>[2x]TNKELQAIRKLLMLDVSEAAEHIGRVSARSWQYWESGRSAVPDDVEQEMLDLASVRIEMMSAIDKRLADGERPKLRFYNKLDEYLADNPDHNVIGWRLSQSVAALYYTEGHADLI

Bacteria are under constant threat of invasion by bacteriophages (phages) and other mobile genetic elements (MGEs). Among the many protection strategies employed against these invaders, the highly diverse CRISPR-Cas systems stand out as the only known adaptive immune systems in bacteria.

Here, we report the first structure of an Aca protein, the Aca2 DNA-binding transcriptional autorepressor from Pectobacterium carotovorum bacteriophage ZF40, determined to 1.34 Å. Aca2 presents a conserved N-terminal helix-turn-helix DNA-binding domain and a previously uncharacterized C-terminal dimerization domain. The elution volume during the final size exclusion chromatography run indicated that the 13.7 kDa Aca2 protein forms a dimer in solution, corroborating what was observed with our previous constructs. The Aca2 dimer structure shows each protomer stacked against one another in opposition, like the letter X, such that the HTH motifs are aligned along the “base” of the dimer. Examining a single protomer shows that the proposed NTD HTH and relative C-terminal domain (CTD) are in fact small clusters of secondary structure elements abutting and joined by a longer backbone α-helix, α4, such that the protomer forms a single globular protein. Whilst the NTD provides the HTH motif for DNA-binding, the CTD stabilizes the positioning of the NTD from the other protomer by stacking α6 against the other protomer α1, thereby aiding dimerization. The Aca2 protomer-protomer interface was analyzed using PDBsum, which calculated a buried surface area of 1213 Å2. This is supported by two salt bridges formed between R57 within α4 of protomer A and E110 within α6 of protomer B, and vice versa. Whilst the upper CTD surface of the dimer contains mixed patches of both electropositive and electronegative potential, the NTD HTH motif is clearly electropositive and primed for DNA binding (left). Dimerization positions the Aca2 recognition helices for insertion into the major grooves of target DNA, supporting its role in regulating anti-CRISPRs.>MAHHHHHHMNATACAPRVRAIVTGHTRGLGASLAEQLLQQDIAVLGVSRSRHPSLAATAGDRLVETELDLSDTAAVAAWLAGGALRSFV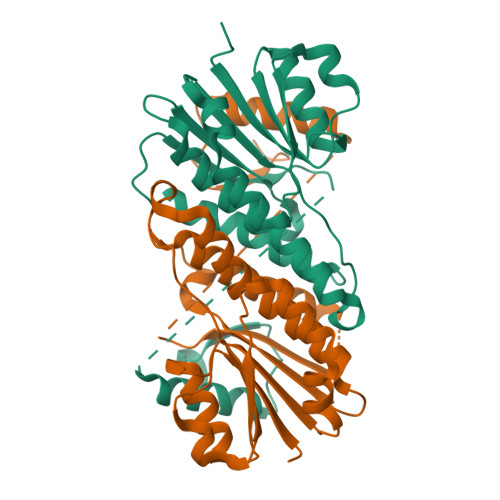DGASLVLLFNNAGVVDPIGPLAAQDPALVARAVALNVAAPLMLSAALVQAAAAPTECRVLHVSSGAARNAYAGWSVYCATKAALDHHARAVALDANRALRICSVAPGVVDTGMQATIRSTSEANFPMREKFDALKASGALSTPDEAARHLIRYALSDAFGAEPTADVRNLPAG[2x]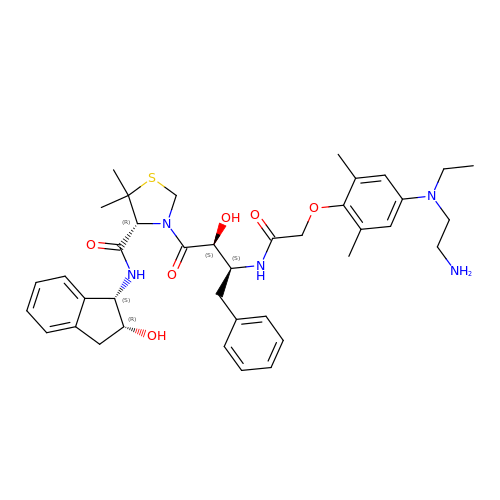(4R)-3-[(2S,3S)-3-[2-[4-[2-azanylethyl(ethyl)amino]-2,6-dimethyl-phenoxy]ethanoylamino]-2-oxidanyl-4-phenyl-butanoyl]-5,5-dimethyl-N-[(1S,2R)-2-oxidanyl-2,3-dihydro-1H-inden-1-yl]-1,3-thiazolidine-4-carboxamide | C39 H51 N5 O6 S | QVEVEYWLPLMZQY-SQKWSBCUSA-N The human telomere contains consecutive repeats of the DNA sequence d[GGGTTA] which can fold into four-stranded intramolecular structures known as G-quadruplexes. The G-quadruplex is a tetra-helical structure formed by guanine-rich sequences, consisting of stacked G-tetrad planes connected by Hoogsteen hydrogen bonds and stabilized by monovalent cations such as Na+ and K+ (4,5). Human telomeric guanine-rich DNA, which could adopt different G-quadruplex structures, plays important roles in protecting the cell from recombination and degradation.

To obtain X-ray diffractive crystals, a double 8Br-dG substitution at 8 and 20 positions in htel21, named as htel21_Br-8,20, was designated for crystallization. The crystal structure of htel21_Br-8,20 was solved by Br-SAD method to ∼1.4 Å resolution in the space group of P6522. The crystal structure shows an intramolecular antiparallel-stranded right-handed chair-type G-quadruplex, comprising three G-tetrad layers in which the hydrogen-bond directionalities of the three G-tetrads are anti-clockwise, clockwise and clockwise (G1←G9←G13←G21, G2→G8→G14→G20 and G3→G7→G15→G19) with all Hoogsteen N1-O6 and N2-N7 hydrogen bonds intact. The glycosidic conformations of guanines around the tetrads are syn•anti•syn•anti. The G-tetrad core are connected by three edgewise side TTA loops. There are three equal-spaced potassium ions, featuring an antiprismatic coordination environment, lying along the axis within the central core of the quadruplex with distance of ∼3.5 Å between K ions. Two of the potassium ions are sandwiched between G-tetrads with an average distance of 2.8 Å from the O6 carbonyl atoms of the guanine residues, while another potassium ion is located between the G3•G7•G15•G19 G-tetrad and T5, T17 with an average distance of 2.9 Å from the O6 carbonyl atoms of the guanine residues and 2.8 Å from the O2 atoms of T5, T17 and the additional two water molecules respectively. The T5 and T17 residues are coplanar with two water molecules stacking on the G-tetrad layer, G3•G7•G15•G19, through a coordinating K+ ion. The A6 and A18 nucleotides form an A6•A18 base pair through N7-N6 hydrogen bonds which caps on coplanar T5, T17 residues. However, it forms a twisted Hoogteen A12•T10 base pair through T10N3-A12N7 and T10O4-A12N6 hydrogen bonds capping on the G1•G9•G13•G21 layer, which partially stabilizes T10 nucleotide.

> GGGTTAGGGTTAGGGTTAGGG> EVVKFMDVYQRSYCHPIETLVDIFQEYPDEIEYIFKPSCVPLMRCGGCCNDEGLECVPTEESNITMQIMRIKPHQGQHIGEMSFL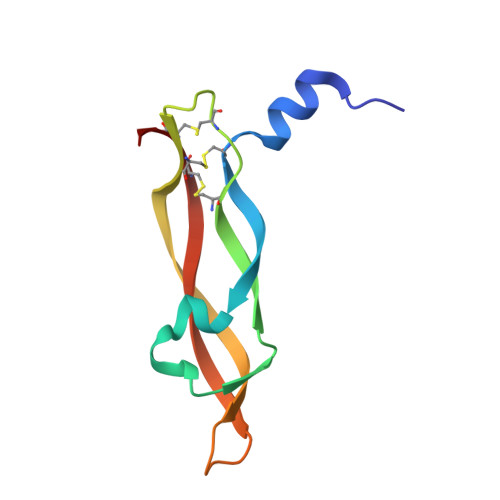QHNKCECRPK> GMPTLEMPVAAVLDSTVGS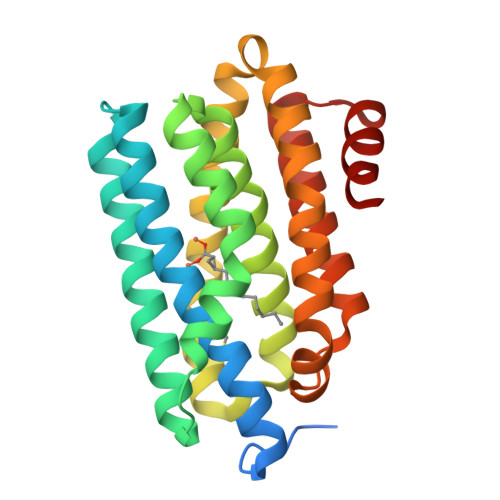SEALPDFTSDRYKDAYSRINAIVIEGEQEAHDNYIAIGTLLPDHVEELKRLAKMEMRHKKGFTACGKNLGVEADMDFAREFFAPLRDNFQTALGQGKTPTCLLIQALLIEAFAISAYHTYIPVSDPFARKITEGVVKDEYTHLNYGEAWLKANLESCREELLEANRENLPLIRRMLDQVAGDAAVLQMDKEDLIEDFLIAYQESLTEIGFNTREITRMAAAALVS> KAQDDSTPDSLFAGLVGEYYGTNSQLNNISDFRALVDSKEADATFEAANISYGRGSSDVAKGTHLQEFLGSDASTLSTDPGDNTDGGIYLQGYVYLEAGTYNFKVT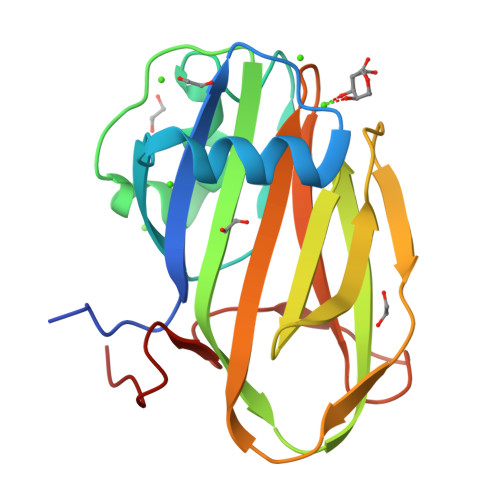ADDGYEITINGNPVATVDNNQSVYTVTHASFTISESGYQAIDMIWWDQGGDYVFQPTLSADGGSTYFVLDSAILSSTGETPYTT>MNHSDTLSLSLELLQQPSVTPIDHTCQTIMADRLAKVGFHI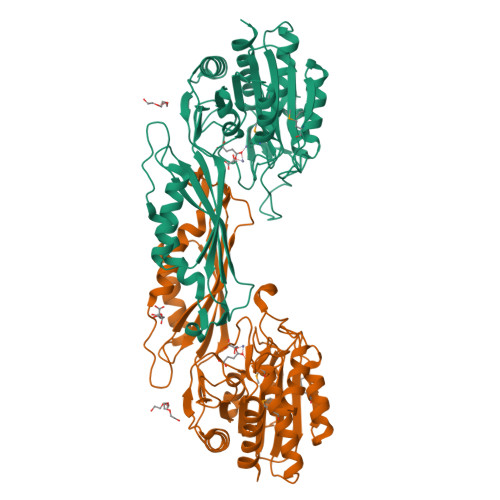EPMRFGDVDNLWARRGTEGPVFCFAGHTDVVPTGRLDAWNSDPFAPEIRDGKLYGRGSADMKTALAAMVVASERFVAKHPNHKGSIAFLITSDEEGPAVNGTVKVIETLEKRNEKITWCLVGEPSSTHKLGDIVKNGRRGSLNAVLKVQGKQGHVAYPHLARNPIHEASPALAELCQTVWDNGNEYFPATSFQISNIHAGTGATNVIPGALEVTFNFRYSTEVTAEQLKQRVHEILDKHGLQYEIVWNLSGLPFLTPVGELVNAAQTAILNVTGTETELSTSGGTSDGRFIAPTGAQVLELGVLNATIHQINEHVDVHDLDPLTDIYEQILENLLAQENLYFQ[2x]> MGSSHHHHHHSQLMVTSTYIPMSQRRSWADVKPIMQDDGPNPVVPIMYSEEYKDAMDYFRAIAAKEEKSERALELTEIIVRMNPAHYTVWQYRFSLLTSLNKSLEDELRLMNEFAVQNLKSYQVWHHRLLLLDRISPQDPVSEIEYIHGSLLPDPKNYHTWAYLHWLYSHFSTLGRISEAQWGSELDWCNEMLRVDGRNNSAWGWRWYLRVSRPGAETSSRSLQDELIYILKSIHLIPHNVSAWNYLRGFLKHFSLPLVPILPAILPYTASKLNPDIETVEAFGFPMPSDPLPEDTPLPVPLALEYLADSFIEQNRVDDAAKVFEKLSSEYDQMRAGYWEFRRRECAEE;> MATEFTPSVYSLVSKPLPSNSRPSATLDEQAETEDLISQLFDLTADPNALVSEHGKRYSGLRKQEHTQFLASSFFQLPGKFVSLDASRPWLVFWTVHSLDLLGVALDQGTKDRVVSTLLHFLSPKGGFGGGPANSQIPHLLPTYASVCSLAIAGNDSSTGGWKDL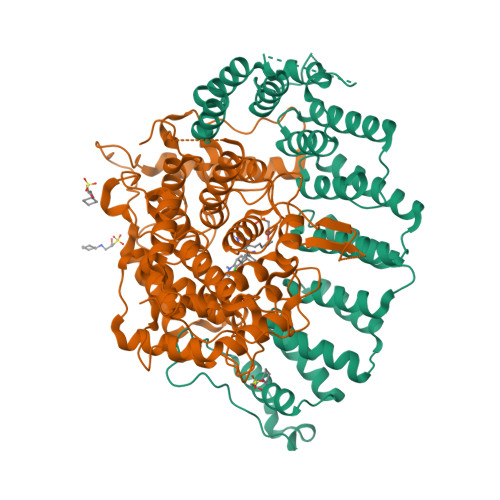AAARQSIYEFFMRCKRPDGGFVVCEGGEVDVRGTYCLLVVATLLDIITPELLHNVDKFVSACQTYEGGFACASFPFPSVVPSTSAFPTSEPSCRVSMAEAHGGYTSCSLNSHFLLTSVPLPSFPLSIDANAALRWTVLQQGEPIEGGGFRGRTNKLVDGCYSWWVGGGAPVAEELVRREKSRKVKKSRIEVFEEEKEGDWEDVPPIPPIFNRVALQEFTLVAAQQDPGSTGGLRDKPGKRPDQYHTCNNLSGLSIAQHKMSHSPSTVSSNRLKFDASKGLPAVKPVAPGGGWKNEDERQNARREIWANALGWIEEEGGEIIVGGKDNRINTTTPVFNILGLRLKPFINYFYCQEN PI3Kδ is a class I PI3K that is formed by a catalytic subunit (p110δ) and a regulatory subunit (p85). Class I PI3Ks catalyze the intracellular conversion of phosphatidylinositol 4,5-bisphosphate (PIP2)2 to phosphatidylinositol 3,4,5-trisphosphate (PIP3), which functions as a second messenger, recruiting and activating signaling proteins such as Akt. Idelalisib (also known as GS-1101, CAL-101, IC489666, and Zydelig) is a PI3Kδ inhibitor that has recently been approved for the treatment of several hematological malignancies. Idelalisib is a potent and selective inhibitor of the kinase activity of PI3Kδ.

The 2.4 Å crystal structure of the idelalisib-PI3Kδ complex showed the inhibitor binding in the ATP-binding site and revealed the specific and entirely noncovalent interactions between inhibitor and protein. Idelalisib binds in the ATP-binding pocket. The purine group of idelalisib serves as the hinge binder, with hydrogen bonds between the purine N3 and the backbone amide of Val-828 and between N9 and the backbone carbonyl oxygen of Glu-826. The purine N7 forms part of a water-mediated hydrogen bond network that includes N1 of the quinazolinone and the side chain of Asp-911. The ethyl group of the inhibitor binds in a hydrophobic pocket formed by Ile-910, Met-900, and Met-752. In the apo enzyme, Met-752 and Trp-760 are packed against each other, but in the presence of idelalisib these two residues lie ∼6.5 Å apart, opening a hydrophobic pocket (the specificity pocket) in which the fluoro-quinazolinone of the inhibitor binds. The phenyl moiety of idelalisib packs against the side chains of Asp-832, Thr-833, and Asn-836. The electron density for idelalisib shows that there is no covalent bond between the inhibitor and the protein. The kinase domain and, in particular the ATP-binding site, is well defined by the electron density, but the Ras-binding and C2 domains have higher temperature factors and are more mobile, as are the residues that link the ABD and the Ras-binding domain. Overall, these observations support the idea that engagement of the specificity pocket upon kinase binding contributes to the selectivity profile of idelalisib.

> GDRVKKLINSQISLLIGKGLHEFDSLRDPEVNDFRTKMRQFCEEAAAHRQQLGWVEWLQYSFPLQLEPSARGWRAGLLRVSNRALLVNVKFEGSEESFTFQVSTKDMPLALMACALRKKATVFRQPLVEQPEEYALQVNGRHEYLYGNYPLCHFQYICSCLHSGLTPHLTMVHSSSILAMRDEQSNPAPQVQKPRAKPPPIPAKKPSSVSLWSLEQPFSIELIEGRKVNADERMKLVVQAGLFHGNEMLCKTVSSSEVNVCSEPVWKQRLEFDISVCDLPRMARLCFALYAVVEKAKKARSTKKKSKKADCPIAWANLMLFDYKDQLKTGERCLYMWPSVPDEKGELLNPAGTVRGNPNTESAAALVIYLPEVAPHPVYFPALEKILELGRHGERGRITEEEQLQLREILERRGSGELYEHEKDLVWKMRHEVQEHFPEALARLLLVTKWNKHEDVAQMLYLLCSWPELPVLSALELLDFSFPDCYVGSFAIKSLRKLTDDELFQYLLQLVQVLKYESYLDCELTKFLLGRALANRKIGHFLFWHLRSEMHVPSVALRFGLIMEAYCRGSTHHMKVLMKQGEALSKLKALNDFVKVSSQKTTKPQTKEMMHMCMRQETYMEALSHLQSPLDPSTLLEEVCVEQCTFMDSKMKPLWIMYSSEEAGSAGNVGIIFKNGDDLRQDMLTLQMIQLMDVLWKQEGLDLRMTPYGCLPTGDRTGLIEVVLHSDTIANIQLNKSNMAATAAFNKDALLNWLKSKNPGEALDRAIEEFTLSCAGYCVATYVLGIGDRHSDNIMIRESGQLFHIDFGHFLGNFKTKFGINRERVPFILTYDFVHVIQQGKTNNSEKFERFRGYCERAYTILRRHGLLFLHLFALMRAAGLPELSCSKDIQYLKDSLALGKTEEEALKHFRVKFNEALRESWKTKVNWLAHNVSKDNRQ> MENTENSVDSKSIKNLEPKIIHGSESMDSGISLDNSYKMDYPEMGLCIIINNKNFHKSTGMTSRSGTDVDAANLRETFRNLKYEVRNKNDLTREEIVELMRDVSKEDHSKRSSFVCVLLSHGEEGIIFGTNGPVDLKK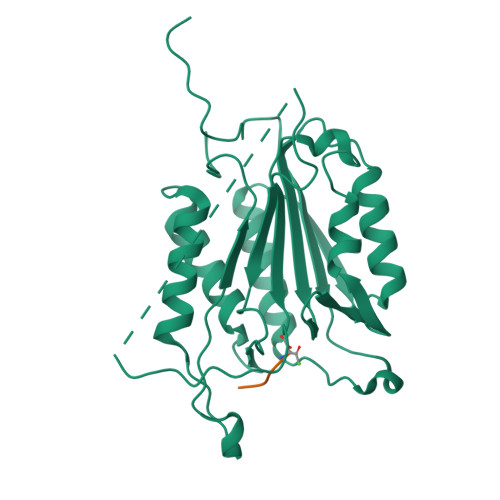ITNFFRGDRCRSLTGKPKLFIIQACRGTELDCGIETDSGVDDDMACHKIPVEADFLYACSTAPGYYSWRNSKDGSWFIQSLCAMLKQYADKLEFMHILTRVNRKVATEFESFSFDATFHAKKQIPCIVSMLTKELYFYH> MNLPTAQEVQGLMARYIELVDVGDIEAIVQMYADDATVEDPFGQPPIHGREQIAAFYRQGLGGGKVRACLTGPV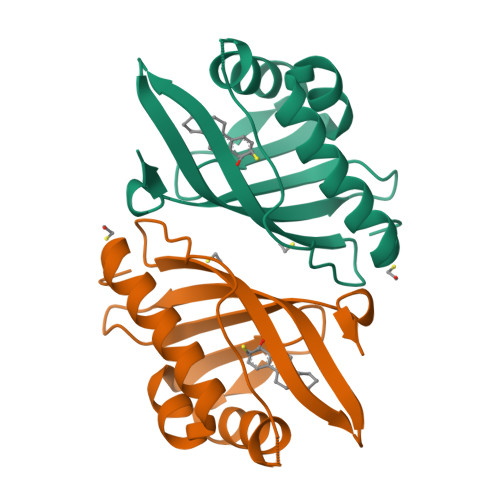RASHNGCGAMPFRVEMVANGQPCALDVIDVMRFDEHGRIQTMQAYWSEVNLSVREPQ>IRAVIYARVSSSDQKEDLERQINYLTNYATAKGYKVVEVLKDIASGLNT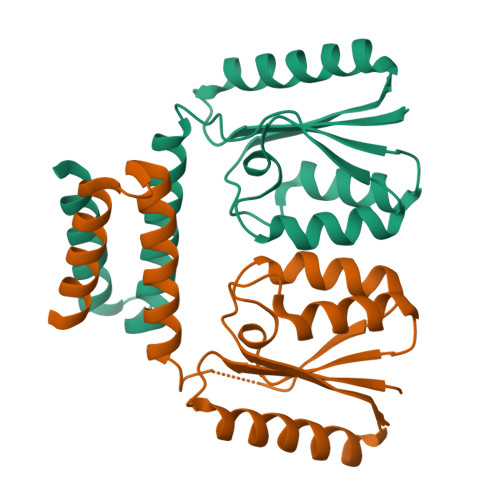QRKGLLKLFKLVEGRSVDVVLITYKDRLTRFGFEYIEELFSTMGVKIEVVFGEEPKDATQELVEDLISIITSFAGKIYGMRSHKKTVLVQGVKKLIGE[4x]In this report, we discovered that XccOpgD, a GH186 homologue from X. campestris pv. campestris, alone converts linear β-1,2-glucan into CβG16α specifically. CβG16α is classified into osmo-regulated periplasmic glucans (OPGs). CβG16α is vital for the pathogenicity toward model plants, Arabidopsis thaliana and Nicotiana benthamiana, despite the nonproduction of CβG16α not affecting the fertility of X. campestris pv. campestris.(3) In detail, CβG16α suppresses the expression of pathogenesis-related (PR) proteins and callose accumulation in plants. Structural analysis of XccOpgD revealed an unprecedented reaction mechanism, anomer-inverting transglycosylation, providing the new concept of the reaction mechanisms among GH enzymes.

The D379N mutant was used to determine a Michaelis complex structure of XccOpgD because D379 is conserved in GH186 and equivalent to the general acid of EcOpgD.12 The complex structure was obtained as a dimer. Three glucan chains were observed in this structure. Two glucans have DPs of 11 and 10 and bind to sites distal from the catalytic pocket of XccOpgD. In the catalytic pockets of the dimer, the electron density of a linear β-1,2-glucan with DP22 was clearly observed only in Chain A (top), probably because the closure motion of the cleft around α-Helix 3 is inhibited by crystal packing in Chain B, implying that the closure motion of the region is needed for substrate recognition. In XccOpgD, the substrate is also observed from subsites −16 to −8. Subsite −16 is located near subsite −1, which appears to be suitable for cyclization. This is consistent with the compound produced by XccOpgD being α-1,6-cyclized β-1,2-glucohexadecaose. Consistently, electron densities at subsites +1 to +6 are obviously observed in the complex structure. In contrast, in XccOpgD, W76 in α-Helix 3 is likely to be important because this residue forms a stacking interaction with the Glc moiety at subsite −16, and this is consistent with the W76A mutant displaying no cyclization activity (<0.1% specific activity compared with wild-type XccOpgD). In XccOpgD, the 6-hydroxy group of the Glc moiety at subsite −16 is located near the anomeric carbon of the Glc moiety at subsite −1.

>[2x]MQRRHFLKNAAAALAALGLPALPPWALAAKAVGLRRLGQPQPFDYAWLKGQARALAKAPYKSHKQVLPGPLESLNWDQYQSIRYRQDHALWADGNGKFQAKFFHLGLYFHTPVHIYDIVDGKAQQLAYDPAAFDYGRSGLGGKQLPKDLGFAGFRLNTRKDTDRDFSAFLGASYFRAVGKEGQYGQSARGLAIDTGTGGPEEFPDFIAYYLEQPADDSDTVVVYGLLDSPSVSGAYRFAITNGEVLVMDIDSALYPRKAIERLGIGPCTSMYQTGENDRRMDWDWRPEIHDTDGLAMWTGGGEWIWRPLCNPPHLRFNMFVDENPRGFGLLQRDRNFDHYQDDGVFYEKRPCLWVEPKSGWGKGSVQLVEIPTVDETFNNIVAFWNPQAKPQPGQELLMGYRLYWGAHPPASSPLAHCVATRTGLGGIVGQKRSHFSWRFAVDFAGGELAALAKDPKAKVEAVLQVSRGTTEIVSARPLHELKGYRAMFDLVPPDEGTQQIDIRLFLRANGKPLTETWLYQWTPPPASERKIYLEHHHHHH>[2x]HHHHHHMIVLFVDFDYFYAQVEEVLNPSLKGKPVVVCVFSGRFEDSGAVATANYEARKFGVKAGIPIVEAKKILPNAVYL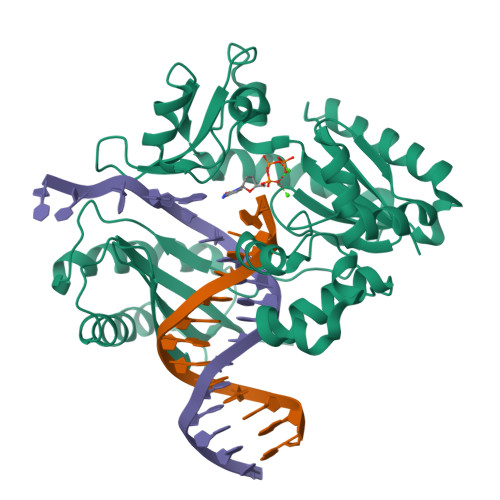PMRKEVYQQVSSRIMNLLREYSEKIEIASIDEAYLDISDKVRDYREAYNLGLEIKNKILEKEKITVTVGISKNKVFAKIAADMAKPNGIKVIDDEEVKRLIRELDIADVPGIGNITAEKLKKLGINKLVDTLSIEFDKLKGMIGEAKAKYLISLARDEYNEPIRTRVRKSIGRIVTMKRNSRNLEEIKPYLFRAIEESYYKLDKRIPKAIHVVAVTEDLDIVSRGRTFPHGISKETAYSESVKLLQKILEEDERKIRRIGVRFSKFIEAIGLDKFFDT> MEKFVLSLDEGTTSARAIIFDRESNIHGIGQYEFPQHYPRPGWVEHNPEEIWDAQLRAIK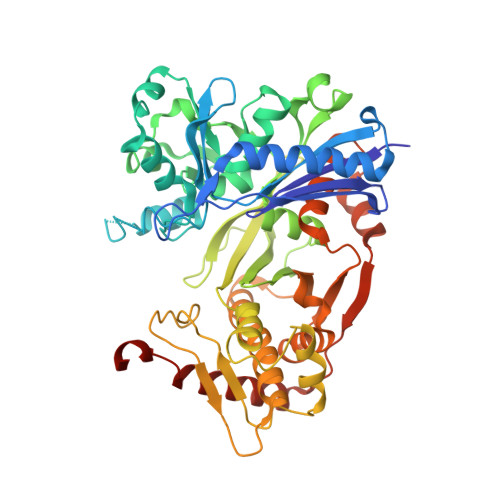DAIQSARIEPNQIAAIGVTNQRETTLVWDKDGKPLYNAIVWQCRRTAEMVEEIKREYGTMIKEKTGLVPDAYFSASKLKWLLDNLPGLREKAEKGEVMFGTVDTFLIYRLTGEHVTDYSNASRTMLFNIKKLDWDDELLELFDIPESVLPEVRESSEVYGYTKKELLGAEIPVSGDAGDQQAALFGEAAFEAGMVKATYGTGSFILVNTDEMVLYSDNLLTTIAWGLNGRVSYALEGSIFVTGAAVQWLRDGIKIIKHASETEELATKLESNEGVYFVPAFVGLGAPYWDQFARGIIIGITRGTGREHLARATLEAIAYLTRDVVDEMEKLVQIKELRVDGGATANDFLMQFQADILNRKVIRPVVKETTALGAAYLAGLAVDYWADTREIAELWKAERIFEPKMDEKTRERLYKGWKEAVKRAMGWAKVVDSAKSN> QVGGV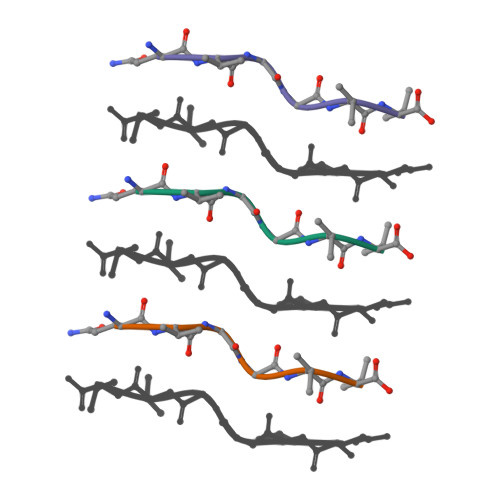V>[2x]GHHHHHHAMSMQDTLLTLDTPAA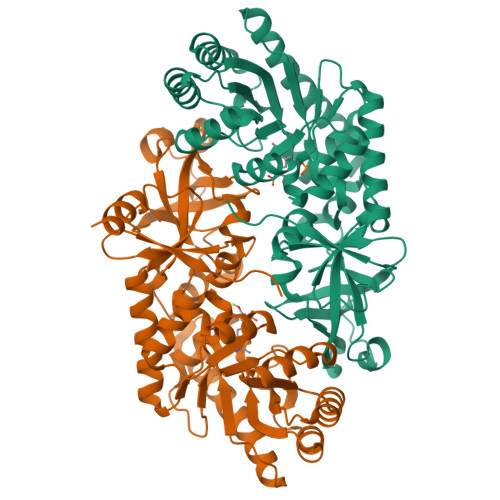VIDLDRMQRNIARMQQRMDAQGVRLRPHVKTSKSVPVAAAQRAAGASGITVSTLKEAEQFFAAGTTDILYAVSMAPHRLPQALQLRRRGCDLKLIVDSVAAAQAIAAFGREQGEAFEVWIEIDTDGHRSGVGADDTPLLLAIGRTLHDGGMRLGGVLTHAGSSYELDTPEALQALAERERAGCVQAAEALRAAGLPCPVVSVGSTPTALAASRLDGVTEVRAGVYVFFDLVMRNIGVCAAEDVALSVLATVIGHQADKGWAIVDAGWMAMSRDRGTARQKQDFGYGQVCDLQGRVMPGFVLTGANQEHGILARADGAAEADIATRFPLGTRLRILPNAACATGAQFPAYQALAADGSVQTWERLHGW>[3x]MAQDWQLSELLENLHADVQHKLTTVRKSFKHSVVKGDGAENVWVDLFNQYLPERYRASRAFVVDSENQFSEQIDVVIYDRQYSPFIFHYAEQLIIPAESVYAVFEVKQTLNKQHIDAARKKV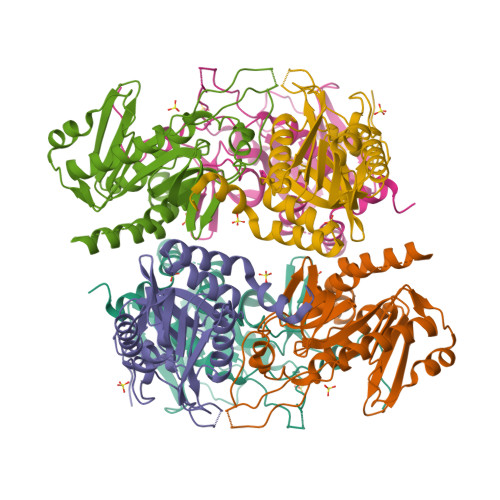ASVRALHRTSLPIPHAGGVHSPRELIGIIGGLLTLENELKIPDTLMGHLDHDKADKGMLNIGCAADDCFFYYDNDHQRMQVMQHKKATTAFLFELLSQLQKCGTVPMIDIHAYGKWLTPRISE> GSTGSMPCPKEDTPNSVWEPAKAKYVFRDVVQITCLDGFEVVEGRVGATSFYSTCQSNGKWSNSKLKCQPVDCGIPESIENGKVEDPESTLFGSVIRYTCEEPYYYMENGGGGEYHCAGNGSWVNEVLGPELPKCVPVCGVPREPFEEKQR;> IIGGSDADIKNFPWQVFFDNPWAGGALINEYWVLTAAHVVEGNREPTMYVGSTSVQTSRLAKSKMLTPEHVFIHPGWKLLEVPEGRTNFDNDIALVRLKDPVKMGPTVSPI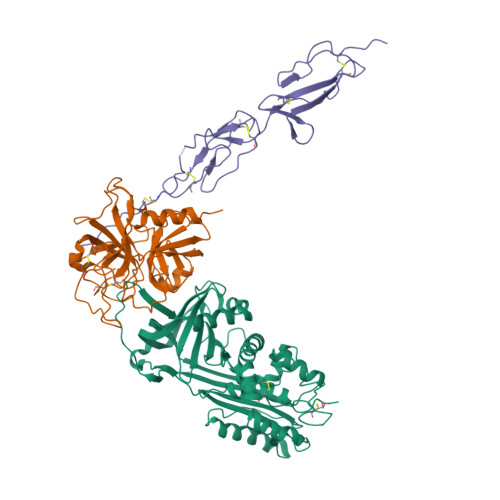CLPGTSSDYNLMDGDLGLISGWGRTEKRDRAVRLKAARLPVAPLRKCKEVKVEKPTADAEAYVFTPNMICAGGEKGMDSCKGDAGGAFAVQDPNDKTKFYAAGLVSWGPQCGTYGLYTRVKNYVDWIMKTMQENSTPRED;> GSTGSTDSPTQPTTGSFCPGPVTLCSDLESHSTEAVLGDALVDFSLKLYHAFSAMKKVETNMAFSPFSIASLLTQVLLGAGENTKTNLESILSYPKDFTCVHQALKGFTTKGVTSVSQIFHSPDLAIRDTFVNASRTLYSSSPRVLSNNSDANLELINTWVAKNTNNKISRLLDSLPSDTRLVLLNAIYLSAKWKTTFDPKKTRMEPFHFKNSVIKVPMMNSKKYPVAHFIDQTLKAKVGQLQLSHNLSLVILVPQNLKHRLEDMEQALSPSVFKAIMEKLEMSKFQPTLLTLPRIKVTTSQDMLSIMEKLEFFDFSYDLNLCGLTEDPDLQVSAMQHQTVLELTETGVEAAAASAISVARTLLVFEVQQPFLFVLWDQQHKFPVFMGRVYDPRA~{N}5-~{tert}-butyl-2-(3-chloranyl-4-fluoranyl-phenyl)-6,7-dihydro-4~{H}-pyrazolo[1,5-a]pyrazine-3,5-dicarboxamide 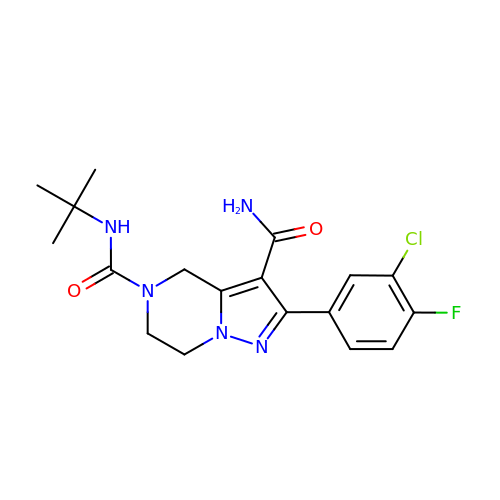| C18 H21 Cl F N5 O2 | PJIBAKKGFKDBLW-UHFFFAOYSA-N>GPLGSHMSTESNDGVSETLLAWRHIDFWTSEHNPDLNATLSDPCTQNDITHAEEDLEVSFPNPVKASFKIHDGQEDLESMTGTSGLFYGFQLMTLDQVVAMTQAWRNVAKNLNKRSQQGLSHVTSTGSSSAMERLNGNKFKLPNIPDQKSIPPNAVQPVYAHPAWIPLITDNAGNHIGVDLAPGPNGKYAQIITFGRDFDTKFVIAENWGEFLLSFANDLEAGNWYLVDDNDDYFSGDGELVFRDKKSNGPIQDYFEVLKRRTWIKYQ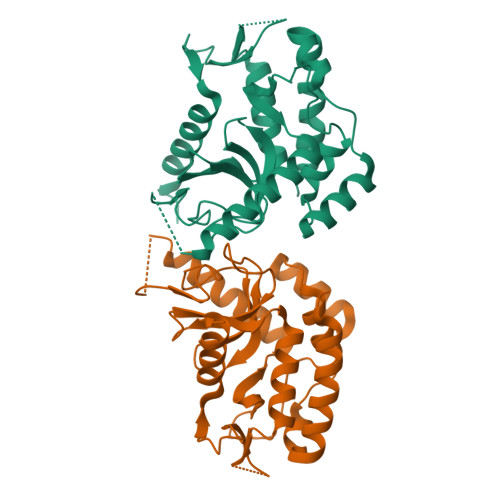LERPHRD[2x]>SNAMTEAMKITLSTQPADARWGEKATYSINNDGITLHLNGADDLGLIQRAARKIDGLGIKHVQLSGEGWDADRCWAFWQGYKAPKGTRKVVWPDLDDAQRQELDNRLMIIDWVRDTINAPAEELGPSQLAQRAVDLISNVAGDRVTYRITKGEDLREQGYMGLHTVGRGSERSPVLLALDYNPTGDKEAPVYACLVGKGITFDSGGYSIKQTAFMDSMKSDMGGAATVTGALAFAITRGLNKRVKLFLCCADNLISGNAFKLGDIITYRNGKKVEVMNTDAEGRLVLADGLIDASAQKPEMIIDAATLTGAAKTA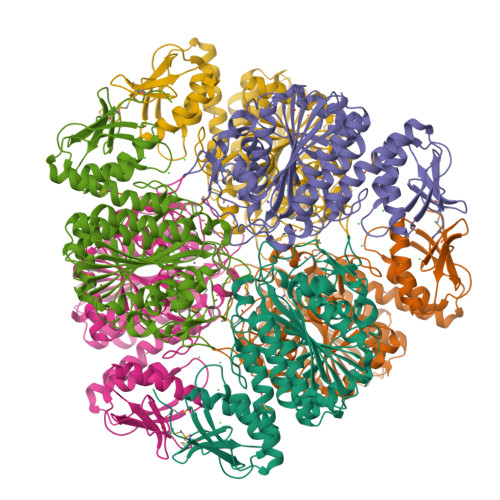LGNDYHALFSFDDALAGRLLASAAQENEPFWRLPLAEFHRSQLPSNFAELNNTGSAAYPAGASTAAGFLSHFVENYQQGWLHIDCSATYRKAPVEQWSAGATGLGVRTIANLLTA[6x]> MAETSEEVAVLVQRVVKDITNAFRRNPHIDEIGLIPCPEARYNRSPIVLVENKLGVESWCVKFLLPYVHNKLLLYRTRKQWLNRDELIDVTCTLLLLNPDFTTAWNVRKELILSGTLNPIKDLHLGKLALTKFPKSPETWIHRRWVLQQLIQETSLPSFVTKGNLGTIPTERAQRLIQEEMEVCGEAAGRYPSNYNAWSHRIWVLQHLAKLDVKILLDELSSTKHWASMHVSDHSGFHYRQFLLKSLISQTVIDSSVMEQNPLRSEPALVPPKDEEAAVSTEEPRINLPHLLEEEVEFSTD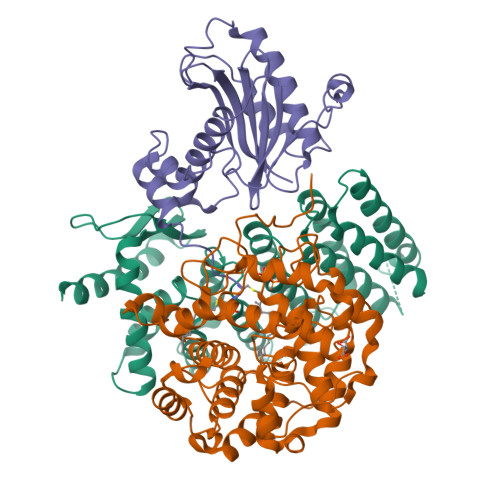LIDSYPGHETLWCHRRHIFYLQHHLN;> GPLGSMGTPQKDVIIKSDAPDTLLLEKHADYIASYGSKKDDYEYCMSEYLRMSGIYWGLTVMDLMGQLHRMNREEILAFIKSCQHECGGISASIGHDPHLLYTLSAVQILTLYDSINVIDVNKVVEYVKGLQKEDGSFAGDIWGEIDTRFSFCAVATLALLGKLDAINVEKAIEFVLSCMNFDGGFGCRPGSESHAGQIYCCTGFLAITSQLHQVNSDLLGWWLCERQLPSGGLNGRPEKLPDVCYSWWVLASLKIIGRLHWIDREKLRNFILACQDEETGGFADRPGDMVDPFHTLFGIAGLSLLGEEQIKPVNPVFCMPEEVLQRVNVQPELVS;> MKLYSLSVLYKGEAKVVLLKAAYDVSSFSFFQRSSVQEFMTFTSQLIVERSSKGTRASVKEQDYLCHVYVRNDSLAGVVIADNEYPSRVAFTLLEKVLDEFSKQVDRIDWPVGSPATIHYPALDGHLSRYQNPREADPMTKVQAELDETKIILHNTMESLLERGEKLDDLVSKSEVLGTQSKAFYKTARKQNSCC>[2x]GPSFWLGNETLKVPLALFALNRQRLCERLRKNPAVQAGSIVVLQGGEETQRYCTDTGVLFRQESFFHWAFGVTEPGCYGVIDVDTGKSTLFVPRLPASHATWMGKIHSKEHFKEKYAVDDVQYVDEIASVLTSQKPSVLLTLRGVNTDSGSVCREASFDGISKFEVNNTIL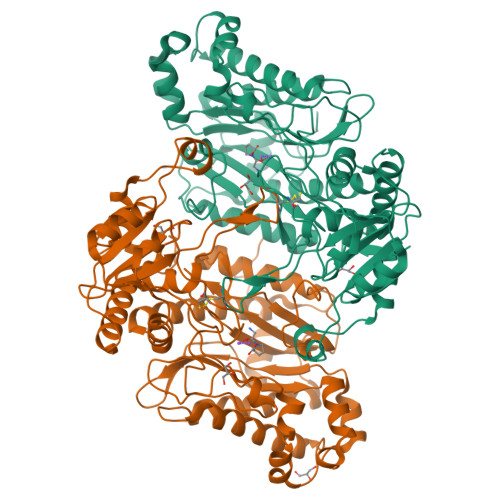HPEIVECRVFKTDMELEVLRYTNKISSEAHREVMKAVKVGMKEYELESLFEHYCYSRGGMRHSSYTCICGSGENSAVLHYGHAGAPNDRTIQNGDMCLFDMGGEYYCFASDITCSFPANGKFTADQKAVYEAVLRSSRAVMGAMKPGVWWPDMHRLADRIHLEELAHMGILSGSVDAMVQAHLGAVFMPHGLGHFLGIDVHDVGGYPEGVERIDEPGLRSLRTARHLQPGMVLTVEPGIYFIDHLLDEALADPARASFLNREVLQRFRGFGGVRIEEDVVVTDSGIELLTCVPRTVEEIEACMAGCDKAFTPF>GSSHHHHHHSSGLVPRGSHMLSVGATTTATRLTGWGRTAPSVANVLRTPDAEMIVKAVARVAESGGGRGAIARGLGRSYGDNAQNGGGLVIDMTPLNTIHSIDADTKLVDIDAGVNLDQLMKAALPFGLWVPVLPGTRQVTVGGAIACDIHGKNHHSAGSFGNHVRSMDLLTADGEIRHLTPTGEDAELFWATVGGNGLTGIIMRATIEMTPTSTAYFIADGDVTASLDETIALHSDGSEARYTYSSAWFDAISAPPKLGRAAVSRGRLATVEQLPAKLRSEPLKFDAPQLLTLPDVFPNGLANKYTFGPIGELWYRKSGTYRGKVQNLTQF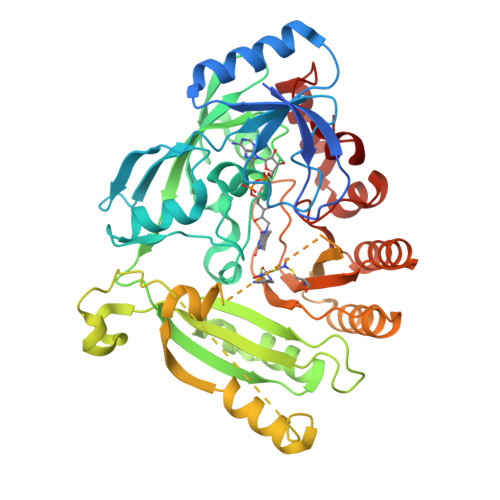YHPLDMFGEWNRAYGPAGFLQYQFVIPTEAVDEFKKIIGVIQASGHYSFLNVFKLFGPRNQAPLSFPIPGWNICVDFPIKDGLGKFVSELDRRVLEFGGRLYTAKDSRTTAETFHAMYPRVDEWISVRRKVDPLRVFASDMARRLELL[2x]>VEDATRSDSTTQMSSTPEVVYSSAVDSKQNRTSDFDANWKFMLSDSVQAQDPAFDDSAWQQVDLPHDYSITQKYSQSNEAESAYLPGGTGWYRKSFTIDRDLAGKRIAINFDGVYMNATVWFNGVKLGTHPYGYSPFSFDLTGNAKFGGENTIVVKVENRLPSSRWYSGSGIYRDVTLTVTDGVHVGNNGVAIKTPSLATQNGGDVTMNLTTKVANDTEAAANITLKQTVFPKGGKTDAAIGTVTTASKSIAAGASADVTSTITAASPKLWSIKNPNLYTVRTEVLNGGKVLDTYDTEYGFRWTGFDATSGFSLNGEKVKLKGVSMHHDQGSLGAVANRRAIERQVEILQKMGVNSIRTTHNPAAKALIDVCNEKGVLVVEEVFDMWNRSKNGNTEDYGKWFGQAIAGDNAVLGGDKDETWAKFDLTSTINRDRNAPSVIMWSLGNEMMEGISGSVSGFPATSAKLVAWTKAADSTRPMTYGDNKIKANWNESNTMGDNLTANGGVVGTNYSDGANYDKIRTTHPSWAIYGSETASAINSRGIYNRTTGGAQSSDKQLTSYDNSAVGWGAVASSAWYDVVQRDFVAGTYVWTGFDYLGEPTPWNGTGSGAVGSWPSPKNSYFGIVDTAGFPKDTYYFYQSQWNDDVHTLHILPAWNENVVAKGSGNNVPVVVYTDAAKVKLYFTPKGSTEKRLIGEKSFTKKTTAAGYTYQVYEGSDKDSTAHKNMYLTWNVPWAEGTISAEAYDENNRLIPEGSTEGNASVTTTGKAAKLKADADRKTITADGKDLSYIEVDVTDANGHIVPDAANRVTFDVKGAGKLVGVDNGSSPDHDSYQADNRKAFSGKVLAIVQSTKEAGEITVTAKADGLQSSTVKIATTAVPGTSTE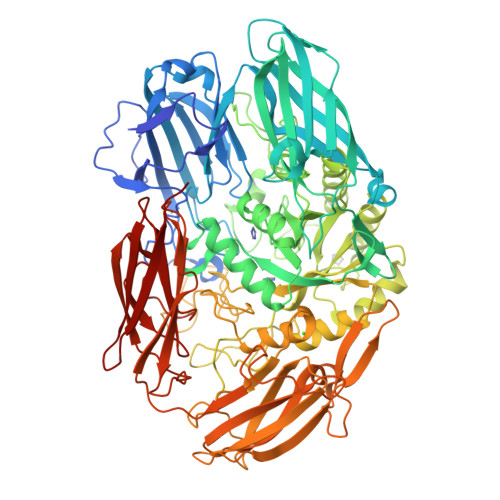[2x]> MQQLQNVIESAFERRADITPANVDTVTREAVNQVIGLLDSGALRVAEKIDGQWVTHQWLKKAVLLSFRINDNKVMDGAETRYYDKVPMKFADYDEARFQKEGFRVVPPATVRQGAFIARNTVLMPSYVNIGAYVDEGTMVDTWATVGSCAQIGKNVHLSGGVGIGGVLEPLQANPTIIEDNCFIGAR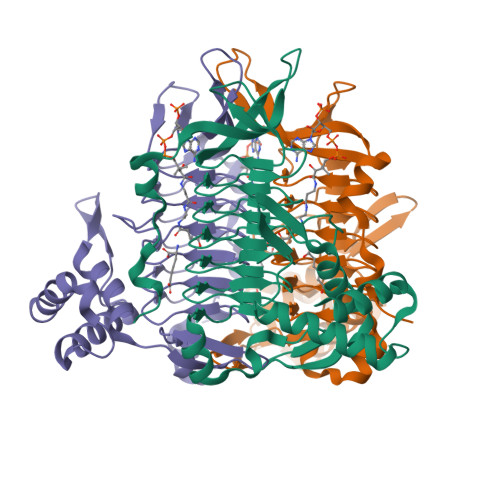SEVVEGVIVEEGSVISMGVYLGQSTRIYDRETGEIHYGRVPAGSVVVSGNLPSKDGSYSLYCAVIVKKVDAKTRGKVGINELLRTID>MSTINNQLKALKVI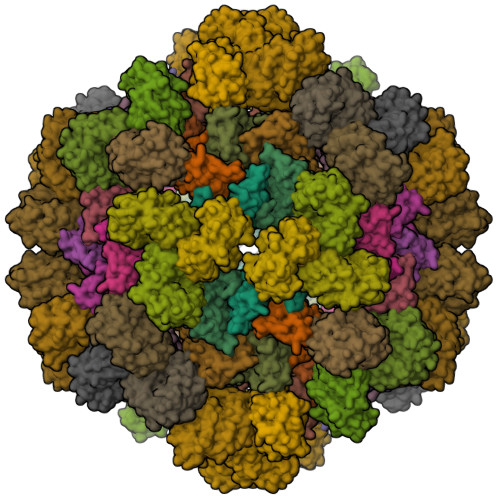PVIAIDNAEDIIPLGKVLAENGLPAAEITFRSSAAVKAIMLLRSAQPEMLIGAGTILNGVQALAAKEAGATFVVSPGFNPNTVRACQIIGIDIVPGVNNPSTVEAALEMGLTTLKFFPAEASGGISMVKSLVGPYGDIRLMPTGGITPSNIDNYLAIPQVLACGGTWMVDKKLVTNGEWDEIARLTREIVEQVNPGSLEHHHHHH[15x];>MTKKVGIVDTTFARVDMASAAILTLKMESPNIKIIRKTVPGIKDLPVACKKLLEEEGCDIVMALGMPGKAEKDKVCAHEASLGLMLAQLMTNKHIIEVFVHEDEAKDDAELKILAARRAIEHALNVYYLLFKPEYLTRMAGKGLRQGFEDAGPARE[15x]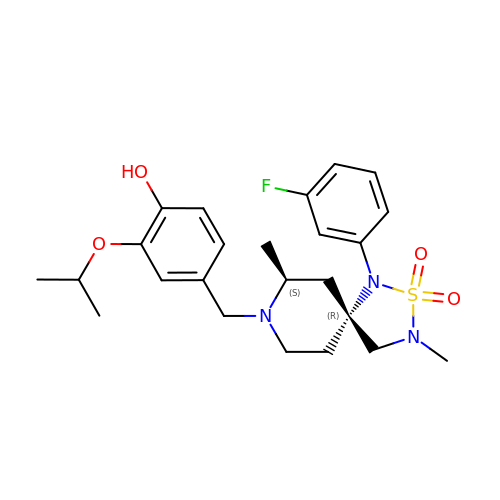4-{[(5R,7S)-1-(3-fluorophenyl)-3,7-dimethyl-2,2-dioxido-2-thia-1,3,8-triazaspiro[4.5]dec-8-yl]methyl}-2-(propan-2-yloxy)phenol | C24 H32 F N3 O4 S | UICGCQDWRACUBV-MHECFPHRSA-N> XRMKQIEDKIEEIESKQKKIE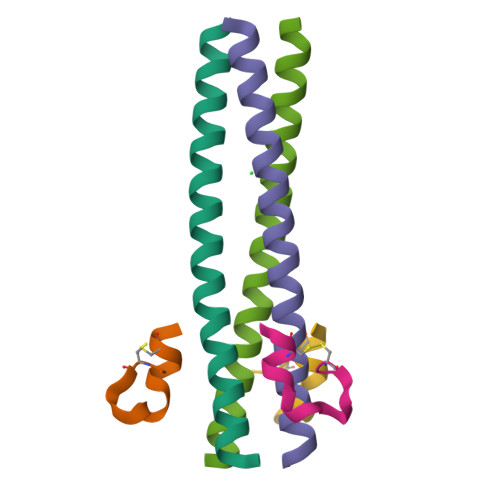NEIARIKKLLQLTVWGIKQLQARIL;> XGACGLGQEEWFWLCAA2,4-DICHLORO-N-(3-CYANO-4,5,6,7-TETRAHYDRO-BENZOTHIOPHEN-2YL)-5-(MORPHOLINE-4-SULFONYL)-BENZAMIDE | C20 H19 Cl2 N3 O4 S2 | 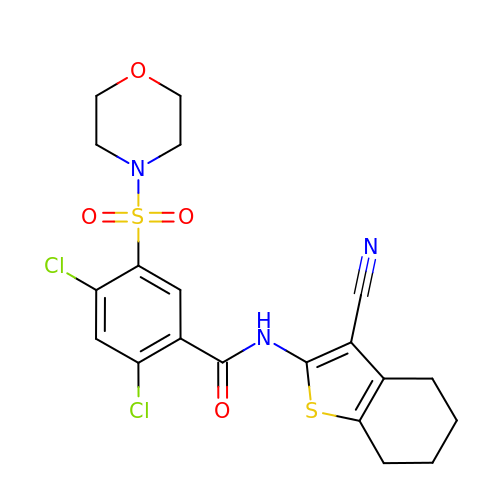JMCVGASJAJMFPN-UHFFFAOYSA-N>MAPLARLAANSARLLQLHKTVPQWHLTDGHLSIKRKFQFSDFNEAWGFMSRVALYADKVDHHP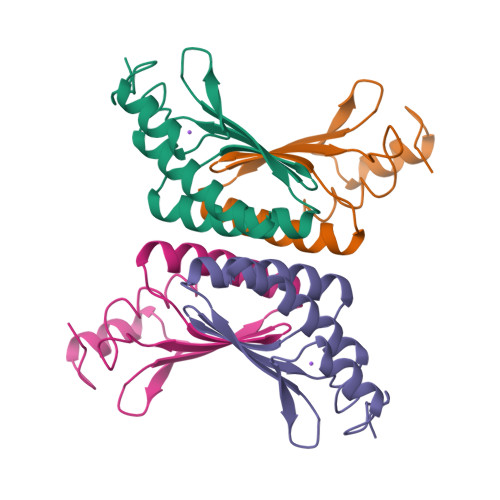NWYNVYNTVDVELSTHDAAGLTEKDFALAKFMDDAAKNFEK[2x]>ASMTGGQQMGRDQAGITGTWYNQLGSTFIVTAGADGALTGTYESAVGNAESRYVLTGRYDSAPATDGSGTALGWTVAWKNNYRNAHSATTWSGQYVGGAEARINTQWLLTSGTTEANAWKSTLVGHDTFTKVKPSA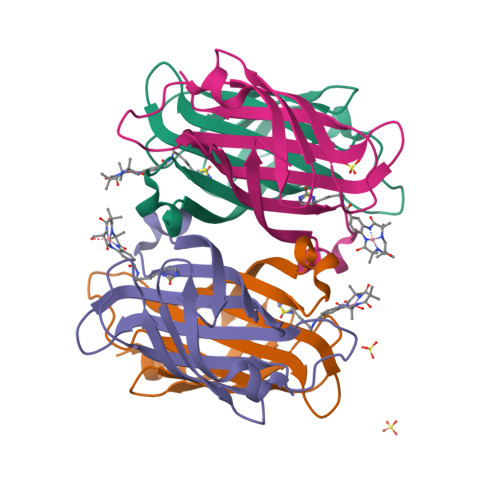ASIDAAKKAGVNNGNPLDAVQQ[4x]2-[[[[(4-CHLORO-6-METHOXY-2-PYRIMIDINYL)AMINO]CARBONYL]AMINO]SULFONYL]BENZOIC 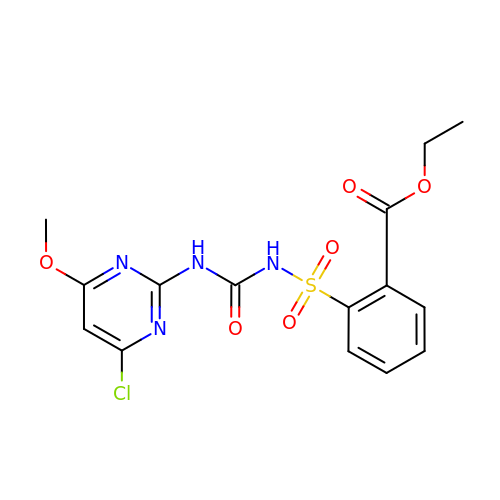ACID ETHYL ESTER | C15 H15 Cl N4 O6 S | NSWAMPCUPHPTTC-UHFFFAOYSA-N Cellulose is synthesized by cellulose synthase (CesA), a membrane-integrated processive family-2 glycosyltransferase (GT; Lombard et al., 2014). The enzyme synthesizes cellulose from UDP-activated glucose (UDP-Glc) and translocates the polymer across the plasma membrane through a channel formed by its own membrane-spanning segment. While bacterial CesAs primarily function as monomeric enzymes, structural analyses of plant CesAs revealed their assembly into triangular-shaped trimeric complexes of three catalytically active subunits. Cryo-EM analyses of all three CesA isoforms reveal the formation of homotrimeric complexes, similar to the secondary cell wall CesAs.

The CSR has been proposed to be intrinsically disordered and only its short N- and C-terminal helical segments are visible in the cryo-EM maps. For GmCesA1, however, at lower contour levels, additional CSR density is evident, extending from corners of the catalytic domains of the GmCesA1 trimer. Viewed from the cytosol, the extra density resembles a hook extending by about 20 Å clockwise and tangentially along the trimer’s corners at the water-lipid interface. At this position, the CSR’s N-terminal conserved cysteine residue(s) postulated to be acylated reside near the membrane interface. The helix has been modeled for GmCesA1 and GmCesA6, while its density is detectable at a similar position but too discontinuous for modeling in the GmCesA3 map. Between the different isoforms, GmCesA1 exhibits greatest product accumulation. In contrast, the activities of GmCesA1 and GmCesA6 peak at pH 8, with a slight decline at pH 9. Quantifying the release of UDP during biosynthesis reactions using a ‘UDP-Glo’ glycosyltransferase assay reveals Michaelis–Menten constants for GmCesA1 and GmCesA3 with respect to UDP-Glc of 0.44 mM and 0.18 mM, respectively. The apparent Vmax value is ~eightfold higher for GmCesA1 compared to GmCesA3. GmCesA1’s apparent IC50 for UDP is about 0.8 mM, whereas this concentration is increased to about 1.3–1.5 mM for GmCesA6 and GmCesA3, respectively.

>MEASAGMVAGSHKRNELVRIRHDSSDSGSKPLKSLNGQICQICGDTVGLTATGDVFVACNECAFPVCRPCYEYERKDGNQSCPQCKTRYKRHRGSPRVEGDEDEDDSDDIENEFNYAQGKAKARRQWEDDADLSSSSRRESQQPIPLLTNGQTMSGEIPCATPDTQSVRTTSGPLGPSEKVHSLPYVDPRQPVPVRIVDPSKDLNSYGLGNVDWKERVEGWKLKQEKNMVQMTGRYTEGKGGDVEGTGSNGEELQMVDDARQPMSRVVPIPSSQLTPYRVVIILRLIILGFFLQYRVTHPVKDAYPLWLTSVICEIWFALSWLLDQFPKWSPINRETYLERLALRYDREGEPSQLDPVDVFVSTVDPLKEPPLVTANTVLSILSVDYPVDKVSCYVSDDGSAMLTFEALSETAEFAKKWVPFCKKHNIEPRAPEFYFAQKIDYLKDKIQPSFVKERRAMKREYEEFKVRINALVAKAQKMPEEGWTMQDGTAWPGNNPRDHPGMIQVFLGHSGGLDTDGNELPRLVYVSREKRPGFQHHKKAGAMNALIRVSAVLTNGAYLLNVDCDHYFNNSKALKEAMCFMMDPVIGKKTCYVQFPQRFDGIDLHDRYANRNIVFFDINMKGQDGVQGPVYVGTGCCFNRQALYGYDPVLTEEDLEPNIIVKSCWGSRKKGKGGNKKYSDKKKAMGRTESTVPIFNMEDIEEGVEGYDDERTLLMSQKSLEKRFGQSPVFIAATFMEQGGIPPSTNPATLLKEAIHVISCGYEDKTEWGKEIGWIYGSVTEDILTGFKMHARGWISIYCMPPRPAFKGSAPINLSDRLNQVLRWALGSIEIFLSRHCPLWYGYNGKLKPLMRLAYINTIVYPFTSIPLIAYCTLPAFCLLTNKFIIPEISNFASMWFILLFVSIFTTSILELRWSGVSIEDWWRNEQFWVIGGTSAHLFAVFQGLLKVLAGIDTNFTVTSKASDEDGDFAELYVFKWTSLLIPPTTVLIVNLVGIVAGVSYAINSGYQSWGPLFGKLFFAIWVIAHLYPFLKGLLGRQNRTPTIVIVWSVLLASIFSLLWVRIDPFTSDSNKLTNGQCGINC[3x]> RPDPTDVFQNKANVCWAKALVPVLKTAGIDMTTEQWNTVDYFETDKAHSAEIVLNQLCVRFFGLDLDSGLFSAPTVPLSIRNN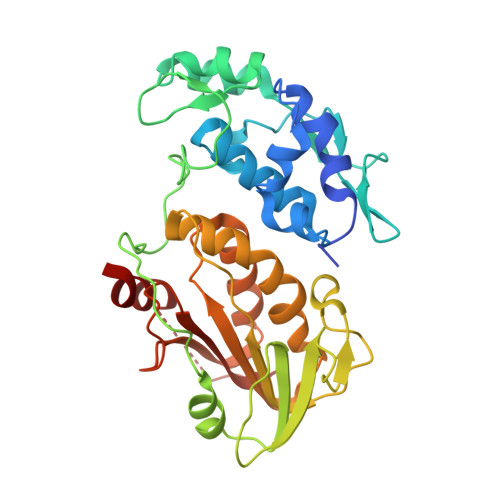HWDNSPSPNMYGLNKEVVRQLSRRYPQLPRAVATGRVYDMNTGTLRNYDPRINLVPVNRRLPHALVLHHNEHPQSDFSSFVSKLKGRTVLVVGEKLSVPGKMVDWLSDRPEATFRARLDLGIPGDVPKYDIIFVNVRTPYKYHHYQQCEDHAIKLSMLTKKACLHLNPGGTCVSIGYGYADRASESIIGAIARQFAFSRVCKPKSSLEETEVLFVFIGYDRAARTHNPYKLSSTLTNIYT>GLYVGGFVDVVSCPKLEQELYLDPDQVTDYLPVTEPLPITIEHLPETEVGWTLGLFQVSHGIFCTGAITSPAFLELASRLADTSHVARAPVKNLPKEPLLEILHTWLPGLSLSSIHPRELSQTPSGPVFQHVSLCA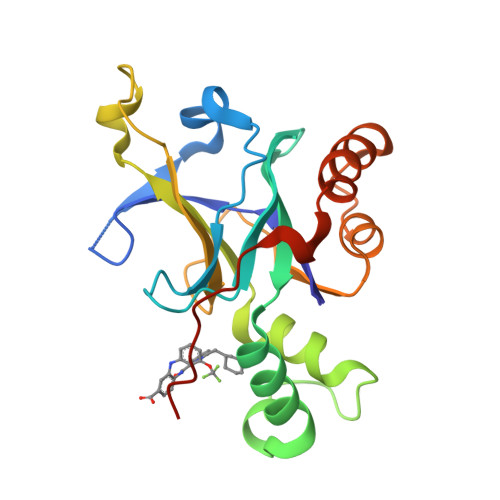LGRRRGTVAVYGHDAEWVVSRFSSVSKSERAHILQHVSSCRLEDLSTPNFVSPLETL[2x]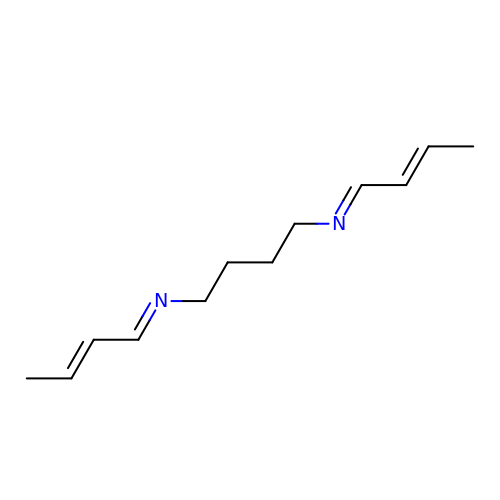N-[(1E,2Z)-but-2-en-1-ylidene]-N'-[(2E)-but-2-en-1-ylidene]butane-1,4-diamine | C12 H20 N2 | GWPFNFBITHRYML-AQVGAVBMSA-N> MTGPTTDADAAVPRRVLIAEDEALIRMDLAEMLREEGYEIVGEAGDGQEAVELAELHKPDLVIMDVKMPRRDGIDAASEIASKRIAPIVVLTAFSQRDL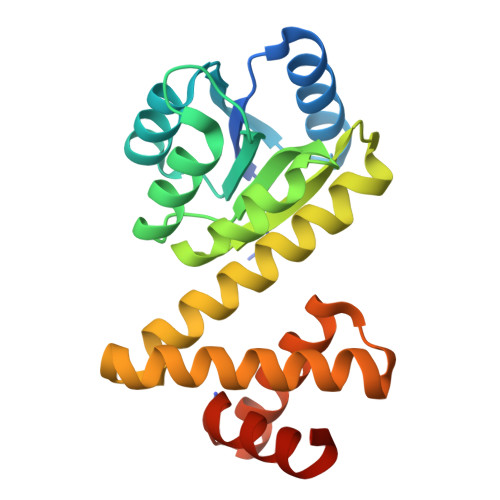VERARDAGAMAYLVKPFSISDLIPAIELAVSRFREITALEGEVATLSERLETRKLVERAKGLLQTKHGMTEPDAFKWIQRAAMDRRTTMKRVAEVVLETLGTPKDT> MNSIFIKNLPTITTRDDILNFFSEVGPIKSIYLSNATKVKYLWAFVTYKNSSDSEKAIKRYNNFYFRGKKLLVTRAQ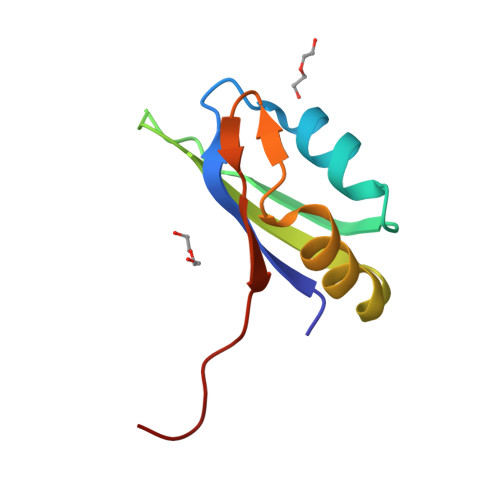DKEERA(3Z)-3-[(4-{[(2S)-2-hydroxy-2-(oxan-4-yl)ethyl]carbamoyl}-3,5-dimethyl-1H-pyrrol-2-yl)methylidene]-2-oxo-N-[(1R)-1-phenylethyl]-3,7-dihydro-2H-indole-5-carboxamide | C32 H36 N4 O5 | 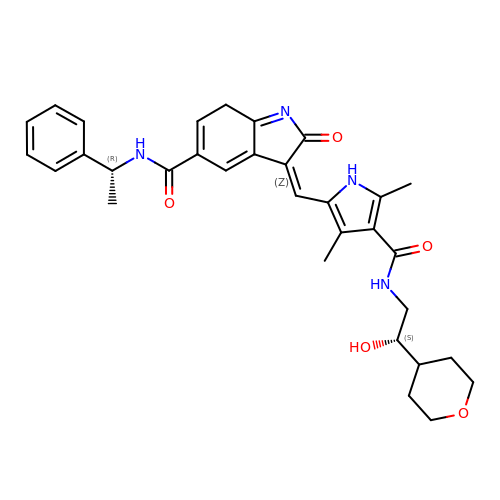ZZTIMXSGQZCALR-SKWDJENRSA-N Strigolactones (SLs) and karrikins (KARs) are two classes of structurally related molecules that mediate signaling pathways to stimulate seed germination. SL and KAR have been reported to be recognized by the homologous proteins D14 (DWARF14)14–17 and HTL (HYPOSENSITIVE TO LIGHT; also known as KAI2, KARRIKIN INSENSITIVE2), respectively. To elucidate the structural basis of ligand specificity, we determined the crystal structures of ShHTL1, ShHTL4, ShHTL7, and ShD14 and compared their structures with those reported for ShHTL331 and ShHTL529. All the structures were highly similar to one another, consisting of a canonical α/β hydrolase domain and a helical cap.

Therefore, our results suggested that ShHTL4, ShHTL7, and ShD14 were able to hydrolyze rac-GR24 and 5DS, but lacked KAR1 binding ability. Y150 was changed to F150 in a subgroup (ShHTL4, ShHTL5, and ShHTL7) of the divergent clade, thus losing the hydrogen bond between helices αD1 and αD3. Therefore, helices αD1 and αD2 of ShHTL4, ShHTL5, and ShHTL7 slid away from αD3, resulting in larger pockets with a reduced chance of causing steric hindrance with ligands. This finding is interesting because ShHTL4, ShHTL5, and ShHTL7 have been shown to be highly sensitive to various natural SLs (polyspecific receptors) in a previous study. ShHTL3 of the intermediate clade evolved from the ancestral HTL paralogs and developed the smallest binding pocket due to the presence of P136 and F190, which are proposed as the major structural bases for the ligand specificity of ShHTL331. It is suggested that the divergent clade ShHTLs lost the ability to bind to KAR due to bulky residue 219, and they developed a highly sensitive subgroup (ShHTL4, ShHTL5, and ShHTL7) for SL binding likely via the evolution of F150 and other pocket-composing residues (e.g., residue 194). ShMAX2 was also able to interact with ShHTL4 of the divergent clade in the presence of rac-GR24. ShHTL4–ShMAX2, ShHTL7–ShMAX2, and ShD14–ShMAX2 interactions were induced in a rac-GR24-dependent manner.

> GPLGSMSTVGSAHNVRVLGSGETTVVLGHGFGTDQSVWKQLVPYLTDEYRVLLYDNMGAGTTNPDCYDFERYSSLEGHSNDLIAILDDFHVTKCIYVGHSLSSMAAAVSSIFRPDLFRKVVMISATPRITNTEDYYGGFEQEEINQMNTAMEENFKTMMMGFAPIVVGGDLESDAIQEFSRTLFNMRPDIALSICRMISGLDLRPYLGLIVVPCHIIQSSKDMLVPVAVAEYLHKNLGGKSVVELIPTEGHLPHLSAPELTIPVLVRHIKHDIA Members of the DAPK family are generally involved in both apoptotic and autophagy pathways and share significant overall sequence similarity with myosin light chain-related kinases and triple functional domain protein-related kinases (Temmerman et al., 2013). DAPK1 and DAPK2 bind Ca2+/CaM through a closely related ARD, which is inhibited by phosphorylation of an identical ARD residue Ser308 in both kinases (Shani et al., 2001, Shohat et al., 2001). They also contain a basic loop (BL) in the kinase N lobe next to the kinase active site, which has been identified as a DAPK-family-specific signature motif (Tereshko et al., 2001). We found an identical type of dimer arrangement in all three kinases that involves the BL of the CD. In terms of functional implications, CD dimerization in hDAPK1, hDAPK2, and hDAPK3 is likely to inhibit catalytic activity by directly occluding the kinase active site.

To explore the molecular mechanisms involved in human DAPK regulation, we expressed and purified truncated versions of hDAPK1, hDAPK2, and hDAPK3. Both the hDAPK1 and hDAPK2 constructs encompass the CD and ARD segments. All three kinases were crystallized and the resulting structures were refined to a resolution of 2.0 Å (hDAPK1), 1.47 Å (hDAPK2), and 3.1 Å (hDAPK3). The dimeric interface areas are in the range of 930–1,600 Å2 in size. This area is smaller in the DAPK1 dimer than in the DAPK2 and DAPK3 dimers, as we were unable to model most of the BL region in this kinase due to weak electron density. By contrast, for hDAPK1 there is a substantially higher level of diversity in terms of possible arrangements. Several other hDAPK1 PDB entries are even monomeric. This is supported by a comparative SEC experiment under the conditions we have established here showing that hDAPK1 tends to be considerably more monomeric than hDAPK2. An analysis of the level of specific dimeric interface interactions indicates an almost complete lack in the hDAPK1 dimer, compared with those found in hDAPK2. Therefore, we speculate that the inhibition of CD-mediated homodimerization of hDAPK1 may have a less pronounced role in regulating hDAPK1 activity than other family members. The highly conserved pattern of four positively charged BL residues in DAPK1 and DAPK2 is suggestive of a common CD-mediated Ca2+/CaM-binding site in both these kinases.

>GTVFRQENVDDYYDTGEELGSGQFAVVKKCREKSTGLQYAAKFIKKRRTKSSRRGVSREDIEREVSILKEIQHPNVITLHEVYENKTDVILILELVAGGELFDFLAEKESLTEEEATEFLKQILNGVYYLHSLQIAHFDLKPENIMLLDRNVPKPRIKIIDFGLAHKIDFGNEFKNIFGTPEFVAPEIVNYEPLGLEADMWSIGVITYILLSGASPFLGDTKQETLANVSAVNYEFEDEYFSNTSALAKDFIRRLLVKDPKKRMTIQDSLQHPWIKPKDTQQALSRKASAVNMEKFKKFAARKKWKQSVRLI[2x]>[4x]SMSGISPKKSKYMTPMQQKLNEVYEAVKNYTDKRGRRLSAIFLRLPSRSELPDYYLTIKKPMDMEKIRSHMMA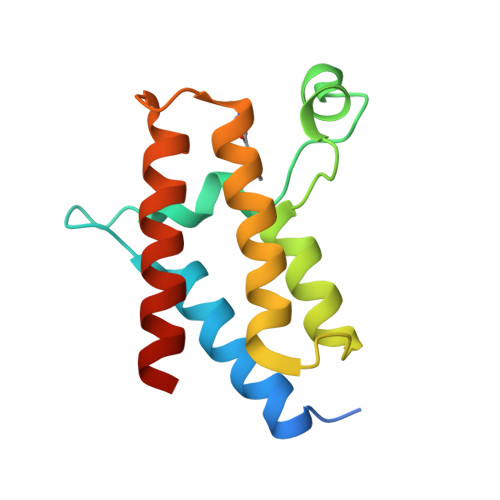NKYQDIDSMVEDFVMMFNNACTYNEPESLIYKDALVLHKVLLETRRDLEGD>[4x]ADPHHHHHHHHAPRPCQAPQQWEGRQVMYQQSSGRNSRALLSYDGLNQRVRVLDERKALIPCKRLFE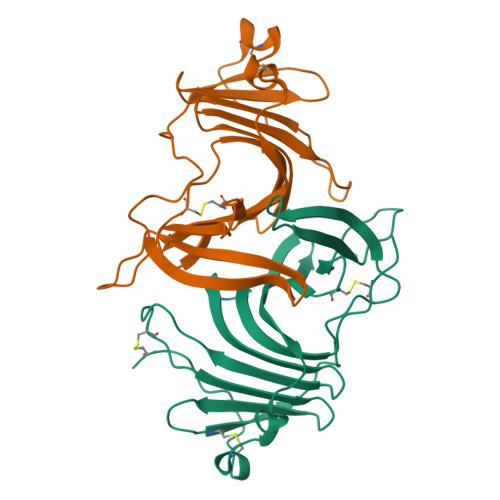YILLYKDGVMFQIDQATKQCSKMTLTQPWDPLDIPQNSTFEDQYSIGGPQEQITVQEWSDRKSARSYETWIGIYTVKDCYPVQETFTINYSVILSTRFFDIQLGIKDPSVFTPPSTCQMAQLEKMSEDCSW RNases H are small nucleases that specifically hydrolyze RNA moieties in various double-stranded nucleic acids that contain both RNA and DNA. Two structural classes of RNases H are designated H1 and H2, and the latter is further divided into RNases H2 and H3 (1,2). Despite the similarity to RNase H2, the type 3 enzyme exhibits the biochemical properties of RNase H1. The RNase H3 N-domain enhances substrate binding and is important for the in vivo function of the enzyme.

Here, we describe the structure of RNase H3 from T. ammonificans complexed with an RNA/DNA hybrid. The best crystals were obtained for Ta-RNase H3 in complex with a 19-mer RNA/DNA and diffracted X-rays to 2.1 Å resolution. In the structure, both domains interact with the RNA/DNA substrate, and the protein covers a continuous stretch of 15 bp of the hybrid. 2′-OH groups of four ribonucleotides, two on each side of the scissile phosphate, interact with the protein, leading to RNA-specific binding: ribonucleotide 5 interacts with the backbone carbonyl of Lys181, ribonucleotide 6 interacts with Glu79, and ribonucleotides 7 and 8 interact with the side chain of Glu84. The scissile phosphate is located at the active site of the enzyme composed of four carboxylates: Asp78 (replaced in the crystallized protein with Asn to inactivate the enzyme), Glu79, Asp180 and Glu206. One metal ion, refined as Mg2+, is observed at the active site, corresponding to metal ion A. It exhibits regular octahedral coordination with six ligands: pro-Sp non-bridging oxygen of the phosphate group of nt 7, pro-Rp oxygen of nt 8, backbone carbonyl of Gly79, side chain of Asn78 and two water molecules. Importantly, the deformation of the substrate 1 nt from the scissile phosphate is observed in RNase H3, which is also a characteristic feature of RNase H2. Our structure explains this by showing that a phosphate group of the DNA strand that is located across the minor groove from the scissile phosphate is bound tightly by the protein, leading to deformation of the non-cleaved strand, which is only allowed for DNA. Therefore, the structure implies that by combining the interactions with the 2′-OH and stacking of aromatic rings with deoxyriboses of the DNA, a relatively small N-domain can achieve specific binding of an RNA/DNA hybrid. In summary, our structure completes the picture of the mechanism of RNases H. RNase H3 represents a notable example of conversion of the substrate specificity from RNA–DNA junction recognition to RNA/DNA hybrid cleavage.

> SMKLSSSEKEKLLKKLKALGAKEEKPPEHAQYRLRLNDAILTVYKSGSVVYGGKGREKLKELVAETVLSDTELPRIGCNEAGKGEFVGPLVVACIVADEKCLKRLIELGVKDSKKLSNEKVEELASEITETCHGKVKLLIPEKYNRAYSKFKNINRLLEAVYREIVSDLCEKFSPKVVVVDKFSNRAEEVLKDVVKGARLEVRPKAEDDLAVAAASIVAKAVRLKTMKELEKRFKVKLPEGNTGLAELLKKTPKELHEKLFKLHFSVGGKK> HMHGRLKVKTSEEQAEAKRLEREQKLKLYQSATQAVFQKRQAGELDESVLELTSQILGANPDFATLWNCRREVLQHLETEKSPEESAALVKAELGFLESCLRVNPKSYGTWHHRCWLLSRLPEPNWARELELCARFLEADERNFHCWDYRRFVAAQAAV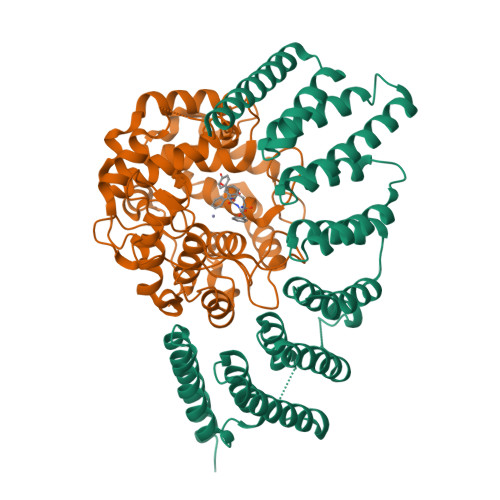APAEELAFTDSLITRNFSNYSSWHYRSCLLPQLHPQPDSGPQGRLPENVLLKELELVQNAFFTDPNDQSAWFYHRWLLGAGSGRCELSVEKSTVLQSELESCKELQELEPENKWCLLTIILLMRALDPLLYEKETLQYFSTLKAVDPMRAAYLDDLRSKFLLENSVLKMEYA;> MGTQQKDVTIKSDAPDTLLLEKHADYIASYGSKKDDYEYCMSEYLRMSGVYWGLTVMDLMGQLHRMNKEEILVFIKSCQHECGGVSASIGHDPHLLYTLSAVQILTLYDSIHVINVDKVVAYVQSLQKEDGSFAGDIWGEIDTRFSFCAVATLALLGKLDAINVEKAIEFVLSCMNFDGGFGCRPGSESHAGQIYCCTGFLAITSQLHQVNSDLLGWWLCERQLPSGGLNGRPEKLPDVCYSWWVLASLKIIGRLHWIDREKLRSFILACQDEETGGFADRPGDMVDPFHTLFGIAGLSLLGEEQIKPVSPVFCMPEEVLQRVNVQPELVS>[4x]MTHHYPTDDIKIKEVKELLP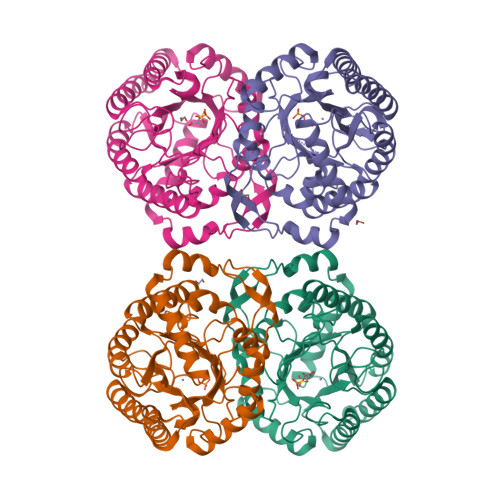PIAHLYELPISKEASGLVHRTRQEISDLVHGRDKRLLVIIGPCSIHDPKAALEYAERLLKLRKQYENELLIVMRVYFEKPRTTVGWKGLINDPHLDGTFDINFGLRQARSLLLSLNNMGMPASTEFLDMITPQYYADLISWGAIGARTTESQVHRQLASGLSCPVGFKNGTDGNLKIAIDAIGAASHSHHFLSVTKAGHSAIVHTGGNPDCHVILRGGKEPNYDAEHVSEAAEQLRAAGVTDKLMIDCSHANSRKDYTRQMEVAQDIAAQLEQDGGNIMGVMVESHLVEGRQDKPEVYGKSITDACIGWGATEELLALLAGANKKRMARAS> MQLSKAAEMCYEITNSYLHIDQKSQIIASTQEAIRLTRKYLLSEIFVRWSPLNGEISFSYNGGKDCQVLLLLYLSCLWEYFFIKAQNSQFDFEFQSFPMQRLPTVFIDQEETFPTLENFVLETSERYCLSLYESQRQSGASVNMADAFRDFIKIYPETEAIV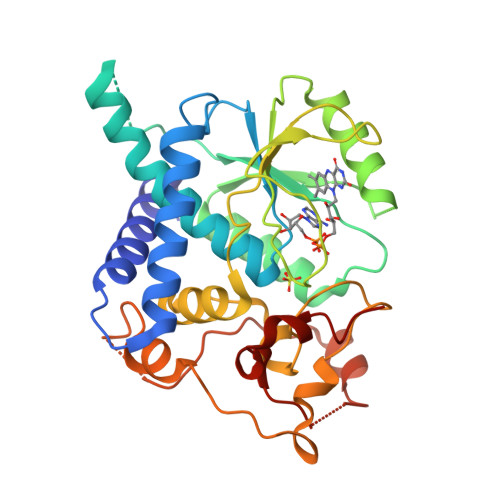IGIRHTDPFGEALKPIQRTDSNWPDFMRLQPLLHWDLTNIWSFLLYSNEPICGLYGKGFTSIGGINNSLPNPHLRKDSNNPALHFEWEIIHAFGKDAEGERSSAINTSPISVVDKERFSKYHDNYYPGWYLVDDTLERAGRIKN> MKEFYLTVEQIGDSIFERYIDSNGRERTREVEYKPSLFAHCPESQATKYFDIYGKPCTRKLFANMRDASQWIKRMEDIGLEALGMDDFKLAYLSDTYNYEIKYDHTKIRVANFDIEVTSPDGFPEPSQAKHPIDAITHYDSIDDRFYVFDLLNSPYGNVEEWSIEIAAKLQEQGGDEVPSEIIDKIIYMPFDNEKELLMEYLNFWQQKTPVILTGWNVESFAIPYVYNRIKNIFGESTAKRLSPHRKTRVKVIENMYGSREIITLFGISVLDYIDLYKKFSFTNQPSYSLDYISEFELNVGKLKYDGPISKLRESNHQRYISYNIIAVYRVLQIDAKRQFINLSLDMGYYAKIQIQSVFSPIKTWDAIIFNSLKEQNKVIPQGRSHPVQPYPGAFVKEPIPNRYKYVMSFDLTSLYPSIIRQVNISPETIAGTFKVAPLHDYINAVAERPSDVYSCSPNGMMYYKDRDGVVPTEITKVFNQRKEHKGYMLAAQRNGEIIKEALHNPNLSVDEPLDVDYRFDFSDEIKEKIKKLSAKSLNEMLFRAQRTEVAGMTAQINRKALINGLAGALGNVWFRYYDLRNATAITTFGQMALQWIERKVNEYLNEVCGTEGEAFVLYGDTDSIYVSADKIIDKVGESKFRDTNHWVDFLDKFARERMEPAIDRGFREMCEYMNNKQHLMFMDREAIAGPPLGSKGIGGFWTGKKRYALNVWDMEGTRYAEPKLKIMGLETQKSSTPKAVQKALKECIRRM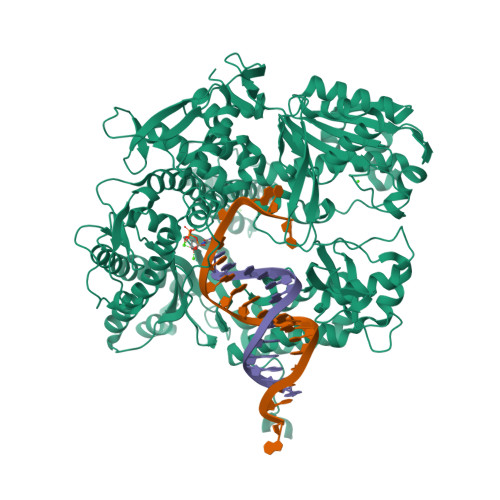LQEGEESLQEYFKEFEKEFRQLNYISIASVSSANNIAKYDVGGFPGPKCPFHIRGILTYNRAIKGNIDAPQVVEGEKVYVLPLREGNPFGDKCIAWPSGTEITDLIKDDVLHWMDYTVLLEKTFIKPLEGFTSAAKLDYEKKASLFDMF> MIRAVFFDSLGTLISVEGAYKVRLKIMEEVLGDYPLNPKTLLDEYEKLAREAFSNYAGKPYRPMRDILEEVMRKLAEKYGFKYPENLREISLRMACRYGELYPEVVEVLKSLKGKYHVGDILQRDTEPATAFLDALGIKDLFDSITTSEEAGFFKPHPRIFELALKKAGVKGEKAVYVGDNPVKDAGGSKNLGMTSILLDRKGEKREFWDKADFIVSDLREVIKIVDELNGQGSLEHHHHHH

SNAr1.3 can operate at a rate of 0.15 s−1, perform more than 4,000 turnovers and can accept a broad range of electrophilic and nucleophilic coupling partners, including those that allow construction of challenging 1,1-diaryl quaternary stereocentres. Biochemical, structural and computational studies provide insights into the catalytic mechanism of SNAr1.3, including the emergence of a halide binding pocket shaped by key catalytic residues Arg124 and Asp125. In summary, we have established a biocatalytic solution to SNAr chemistry, one of the most important classes of transformations in the chemical industry.

Notably, iodide was found to be a more potent inhibitor of SNAr1.3, with an IC50 value of 1.20 ± 0.05 mM. The resulting structure reveals two internal iodide binding sites, with the most occupied site (about 85%) shaped by Met64, Arg65, Arg124, Asp125 and Pro128. Notably, Arg and Asp residues are a common feature of halide binding sites in natural proteins, despite the latter being negatively charged. Guided by the structural analysis, we performed site-directed mutagenesis of residues lining the halide binding site. R124A and D125N/A mutations led to substantial 180-fold and 68-fold/22-fold reductions in rate, respectively, with more modest 5.4-fold and 10-fold rate reductions observed with M64A and R65A. These assays further underscore the importance of the halide binding motif to efficient catalysis, although the large contribution made by Arg124 could also be ascribed to its role in nucleophile activation (vide infra). Notably, although high levels of selectivity were preserved with the M64A, R65A and D125A halide cavity mutations, the R124A mutation led to a substantial loss of enantioselectivity, suggesting that Arg124 may also play a role in positioning and/or activating the nucleophile 1 for selective catalysis. This hypothesis is supported by molecular dynamics simulations that reveal productive conformations with the enolate of 1 forming hydrogen bonding interactions with Arg124.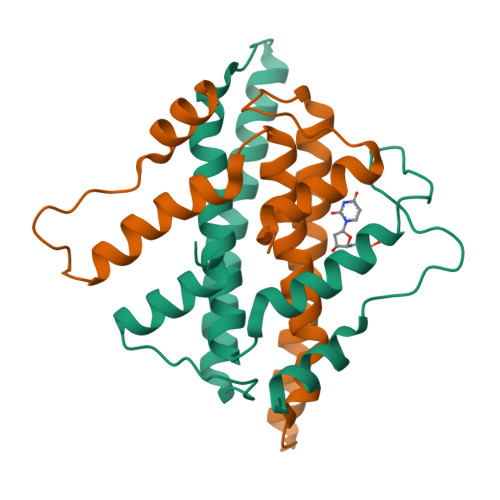>[4x]PPTNAERLHEFHRAIGAATPERPTPPPPELLRLRQTLLDAESAEVRAEIDHLLARQAAGEALSAGDLAPLAHELADLLYVTYGALDQLGIDADAVFAEVHRANLSKASGPRRADGKQLKPEGWRPADVRGVIERLQHA>QQFPNECQLDQLNALEPSHVLKAEAGRIEVWDHHAPQLRCSGVSFVRYIIESKGLYLPSFFSTAKLSFVAKGEGLMGRVVPGCAETFQDSSVFQPGGGSPFGEGQGQGQQGQGQGHQGQGQGQQGQQGQQGQQSQGQGFRDMHQKVEHIRTGDTIATHPGVAQWFYNDGNQPLVIVSVLDLASHQNQLDRNPRPFYLAGNNPQGQVWIEGREQQPQKNILNGFTPEVLAKAFKIDVRTAQQLQNQQDNRGNIIRVQGPFSVIRPPLRSQRPQEEVNGLEETICSARCTDNLDDPSNADVYKPQLGYISTLNSYDLPILRFL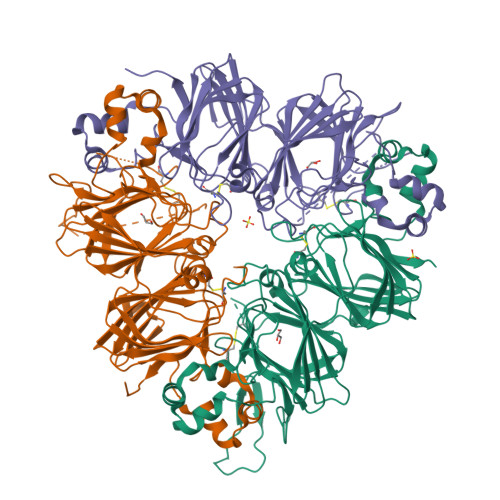RLSALRGSIRQNAMVLPQWNANANAVLYVTDGEAHVQVVNDNGDRVFDGQVSQGQLLSIPQGFSVVKRATSEQFRWIEFKTNANAQINTLAGRTSVLRGLPLEVISNGYQISLEEARRVKFNTIETTLTHSSGPASYGGPRKADA[6x]>[2x]MQSPPPDPLGDCLRNWEDLQQDFQGIQETHRLYRLKLEELTKLQANCTNSITRQKKRLQELALVLKKCRPSLPSESMEAAQEL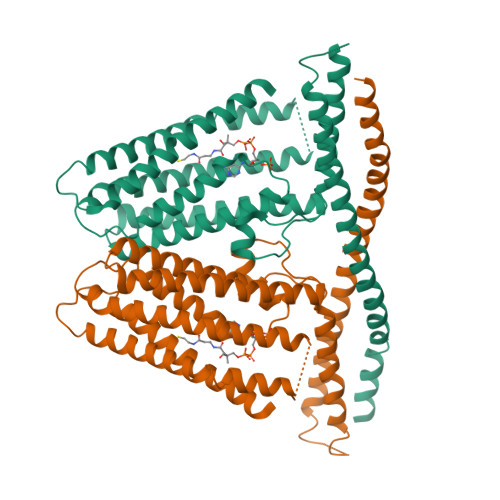ENQMKERQGLFFDMEAYLPKKNGLYLSLVLGNVNVTLLSKQAKFAYKDEYEKFKLYLTIILIVISFTCRFLLNSRVTDAAFNFLLVWYYCTLTIRESILINNGSRIKGWWVFAAYVSTFLSGVMLTWPDGLMYQKFRNQFLSFSMYQSFVQFLQYYYQSGCLYRLRALGERHTMDLTVEGFQSWMWRGLTFLLPFLFFGHFWQLFNALTLFNLARDPECKEWQVLMCGFPFLLLFLGNFFTTLRVVHQKFHSQQHGNKKD> MSSLRLVSSSTIQAANDNNDDSSQLIDLTVWDLIGLERESIQQGLLYHHPNQ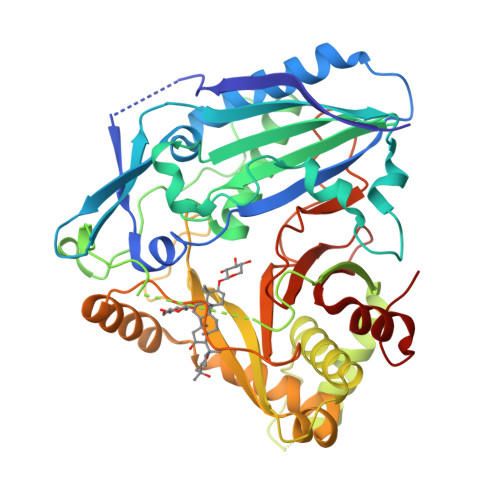VDTPNQIQHLKHSLSSTLSFFPPFAGRLVITEYEDNTATCFIACNNAGALFVHAVAENTTISDILQPNKYVPPIVNSLFSLNGVKNREGTIQPLLVVQVTELVDGIFIGLTVNHVVADGKSFWLFVNSWAEISRGFQKPSKLPTLERWFLNDTDHPIRFSFSMEEEKKKFQSGQLTTRFFHFTRENIAHLKSKANGEVTLGNTERRISSLQALLAHVWRSVVRCERIDPQEVLYYILLIDARTRLIPPLEDDYFGNAADAGVVIMKAGELLEGGLGNVAWNMNKVISLNSDEKIKNRYKSWLRTPQLPSMGMHTTFASQLLIIANSPRFNVYGNDFGWGKPLAVRSSAENKRDCKIVLFAGAEEGSIDIEVCLPYEILEALGNDAEFLDNHSIG>MGSSHHHHHHSSGLVPAGSHMRRTQQGTTASPPVLDLGALGQDFAADPYPTYARLRAEGPAHRVRTPEGNEVWLVVGYDRARAVLADPRFSKDWRNSTTPLTEAEAALNHNMLESDPPRHTRLRKLVAREFTMRRVELLRPRVQEIVDGLVDAMLAAPDGRADLMESLAWPLPITVISELLGVPEPDRAAFRVWTDAFVFPDDPAQAQTAMAEMSGYLSRLIDSKRGQDGEDLLSALVRTSDEDGSRLTSEELLGMAHILLVAGHETTVNLIANGMYALLSHPDQLAALRADMTLLDGAVE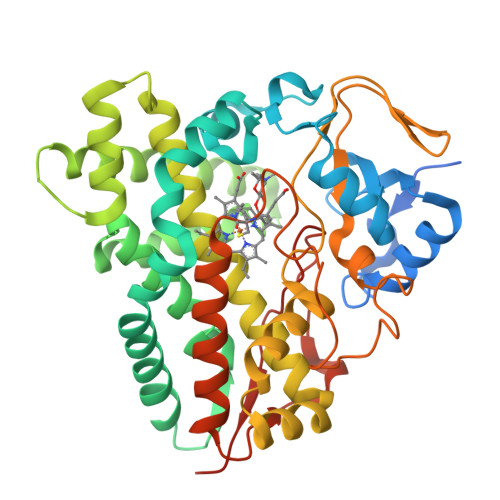EMLRYEGPVESATYRFPVEPVDLDGTVIPAGDTVLVVLADAHRTPERFPDPHRFDIRRDTAGHLAFGHGIHFCIGAPLARLEARIAVRALLERCPDLALDVSPGELVWYPNPMIRGLKALPIRWRRGREAGRRTG[2x]> GISCSDPNPLDSYTRVPFEKTETDDGNGDGDGDGAGGLFEKGNGTDSKPYMIMNATQIRNMRSVLKSGMKVYFQLGADIDMAGIDDWQSLNGSGDFPYEIDFDGDSHVIKNFKCSAGDYPSFFGVLCGDCRNVGFVNASVSSARQGIGI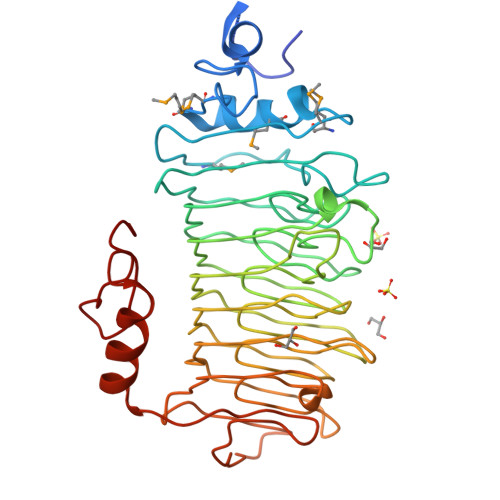ITGYLGLKDKGNGNKTGRIVNCYTTGEVIGSGAAGGIAGVLANSYDGQESYIKNCYSNATVSDRAASGGKAGGIAGRKVGVGGFIENCYAYGAVSATKGGVGGILGQIDKSCDIAIKNSAAWSNLTGVDASSTVGRIVGVSASLGSYENCYACESIVLKVNEKTITASDESSATGTTFHGVAKSAEELGNIIVAWNPNLWKKGTNGYPIFQWSE> GRPAGMQAVKSPSEAGALQLVELNGQLTLAGEDGTPVQLRGMSTHGLQWFGEIVNENAFVALSNDWGSNMIRLAMYIGENGYATNPEVKDLVYEGIELAFEHDMYVIVDWHVHAPGDPRADVYSGAYDFFEEIADHYKDHPKNHYIIWELANEPSPNNNGGPGLTNDEKGWEAVKEYAEPIVEMLREKGDNMILVGNPNWSQRPDLSADNPIDAENIMYSVHFYTGSHGASHIGYPEGTPSSERSNV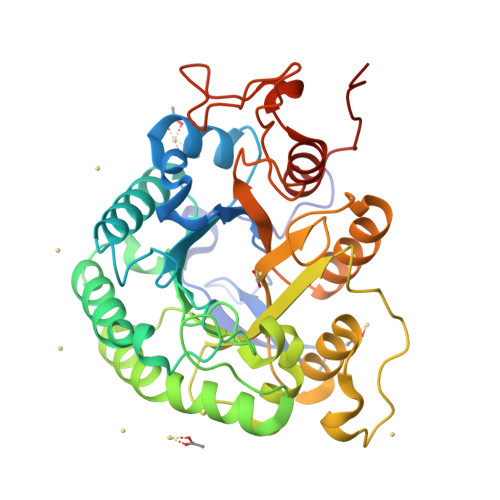MANVRYALDNGVAVFATEWGTSQANGDGGPYFDEADVWLNFLNKHNISWANWSLTNKNEISGAFTPFELGRTDATDLDPGANQVWAPEELSLSGEYVRARIKGIEYTPIDRTKFTKL methyl [(1E,5R)-5-{(3S)-3-[(2E,4E)-2,5-dimethylocta-2,4-dienoyl]-2,4-dioxo-3,4-dihydro-2H-pyran-6-yl}hexylidene]carbamate | C23 H31 N O6 | 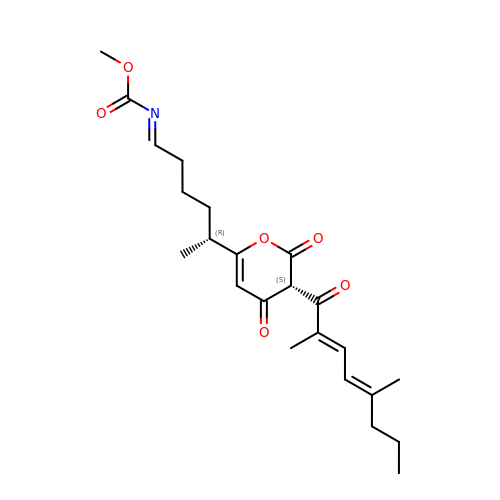LTDLIPXLSBMTFP-FSAISGGASA-N> SVTVKRIIDNTVIVPKLPANEDPVEYPADYFRKSKEIPLYINTTKSLSDLRGYVYQGLKSGNVSIIHVNSYLYGALKDIRGKLDKDWSSFGINIGKAGDTIGIFDLVSLKALDGVLPDGVSDASRTSADDKWLPLYLLGLYRVGRTQMPEYRKKLMDGLTNQCKMINEQFEPLVPEGRDIFDVWGNDSNYTKIVAAVDMFFHMFKKHECASFRYGTIVSRFKDCAALATFGHLCKITGMSTEDV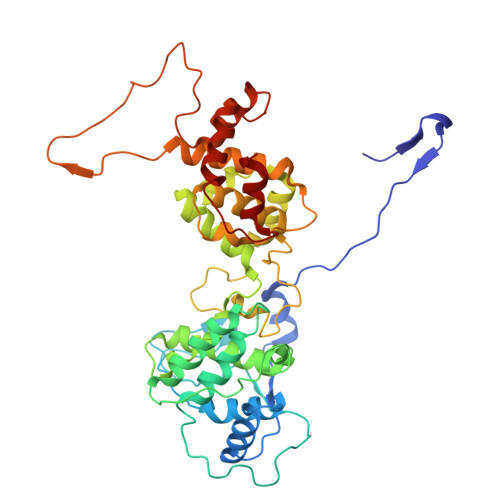TTWILNREVADEMVQMMLPGQEIDKADSYMPYLIDFGLSSKSPYSSVKNPAFHFWGQLTALLLRSTRARNARQPDDIEYTSLTTAGLLYAYAVGSSADLAQQFCVGDNKYTPDDSTGGLTTNAPPQGRDVVEWLGWFEDQNRKPTPDMMQYAKRAVMSLQGLREKTIGKYAKSEFDK> MSDLVNKKFPAGDYKFQYIAISQSDADSESCKMPQTVEWSKLISENKKVIITGAPAAFSPTCTVSHIPGYIN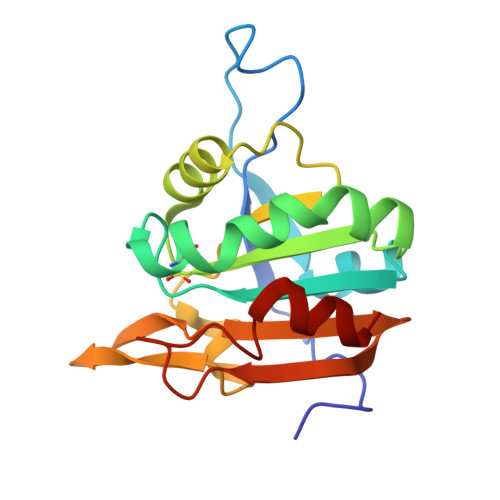YLDELVKEKEVDQVIVVTVDNPFANQAWAKSLGVKDTTHIKFASDPGCAFTKSIGFELAVGDGVYWSGRWAMVVENGIVTYAAKETNPGTDVTVSSVESVLAHL5'-O-[N-(L-TYROSYL)SULFAMOYL]ADENOSINE | C19 H23 N7 O8 S | 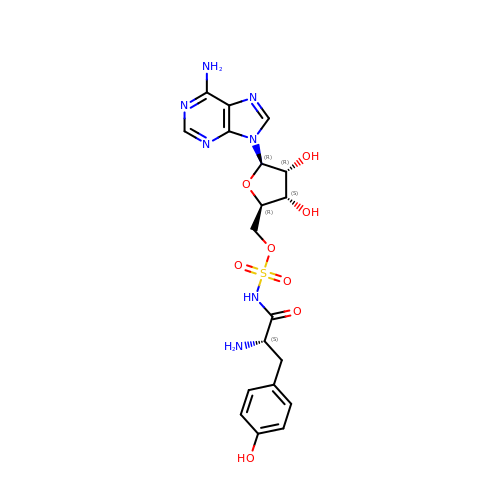MJZAZMKENKZBAJ-QTOWJTHWSA-N>MSERHLFTSESVSEGHPDKIADQISDAILDAMLAQDPQARVAVETSVTTGLVLVFGEVSTKAYVDIQKVVRDTIKSIGYVDGQYGFDGDNCAVLVSLDEQSPDIAQGVDDSLETRSGDADPLDQIGAGDQGMMFGYAINETPELMPLPIALSHRLMRKIAALRKDGTIKWLRPDAKAQVTVEYDEDNQPKRIDTVVLSTQHDPDVDLDTIRQTVIDQVIKAVLPADLLDDQTKYLVNPTGRFVIGGPQGDAGLTGRKVIVDTYGGFAHHGGGAFSGKDATKVDRSASYAARYIAKNVVAAGLADQVEVQLAYAIGVAEPVSIAVDTAGTGKVSDEALINAIRENFDLRPAGIIKMLDLQRPIYRQTAAYGHFGRTDIDLPWEHTDKVDALKAAF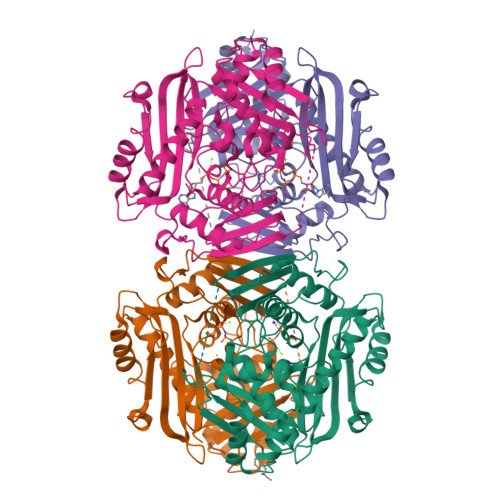KHHHHHH[8x]> MASWSHPQFEKGAMQPTAIRSTVGLPGADMTADLRDPAPVAVPAHSAADAAAPPPGALQTIVGRPPRPDGPRHRRAQSLPARLTPAQRGMLAELGVADTSVLTPTETAVLRELRLHRPPLPLDTLLFTDPNKDPDDVVTYTIAKQLQAEGFLRLTDVVVTLGDADMRSQRAQLAKGVFDRLALPEVRVARGQDYPMTSTQAREHSKFLAEGAALRAAPDAVHTDGVRAMRERLATSPHKLGMVVIAGMTDASALLAEAGDLVREKL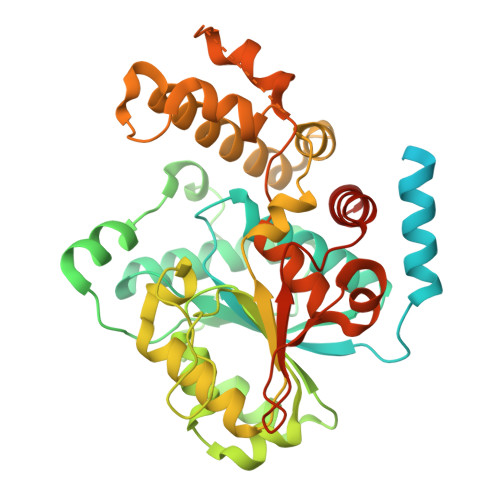ASITIMGGIDPARDADGLVQPDTRAYNNATDIHAARALYRRAQQLGIPLRILSKEAAYRAAVPPAFYEGIARNGHPVGEYLRDVQKNALKGLWEGIQANLIPGLDTAWFFRTFVAAQPQDPAAADQQGAMSFDAIWPQVTKLNLYDPLTLLAALPGAARLLFQPTPMHREGASPVEHVGHAEVVRPEKARLLLSALAKAALAQQDEGQRGR>G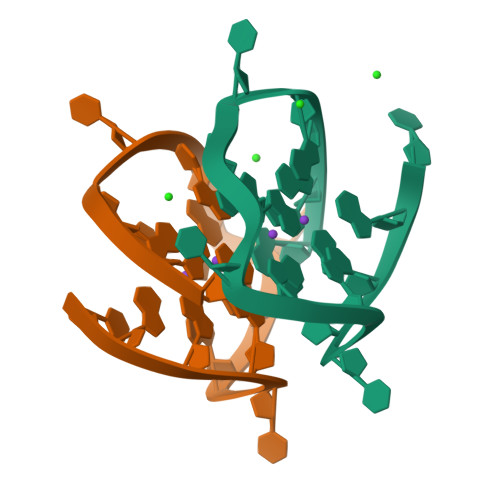GGGTGGGCGGTGGGT[2x]> GPSSTVTIEYFNQKKEMTKTLEEITRDFEKENPKIKVKVVNVPNAGEVLKTRVLAGDVPDVVNIYPQSIELQEWAKAGVFEDLSNKDYLKRVKNGYAEKYAVNEKVYNVPFTANAYGIYYNKDKFEELGLKVPETWDEFEQLVKDIVAKGQTPFGIAGADAWTLNGYNQLAFATATGGGKEANQYLRYSQPNAIKLSDPIMKDDIKVMDILRINGSKQKNWEGAGYTDVIGAFARGDVLMTPNGSWAITAINEQKPNFKIG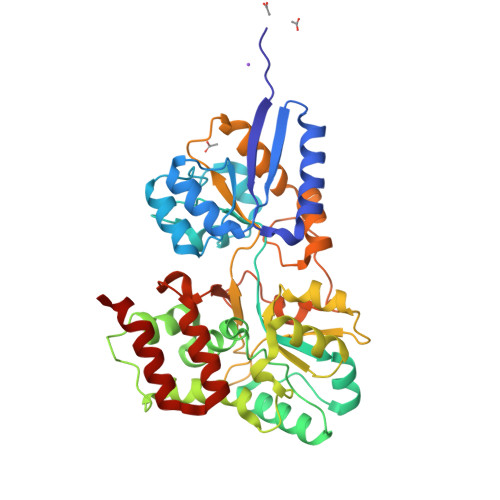TFMIPGKEKGQSLTVGAGDLAWSISATTKHPKEANAFVEYMTRPEVMQKYYDVDGSPTAIEGVKQAGEDSPLAGMTEYAFTDRHLVWLQQYWTSEADFHTLTMNYVLTGDKQGMVNDLNAFFNPMKM> GAEVGRLRYPPEMPGAEVKVYKKVDNVDLKLYIYKPADWKPADRRSAIVFFFGGGWQSGSPAQFRPQCEYFAGRGMVAMAADYRVGSRHNVKVADCVADAKSAIRWVRQHAAELGVDPQKIVASGGXAGGHLAACTVMVPDLEAPEEDHTISSQANAAILFNPVLILSREGLKDHVPRQDWEERLRERLGTEPKAVSPYHHIRAGLPPMIIFHGTADNTVPFETIRLFAEAMKKAGNRCELVPFEGAAHGFFNFGRGDNLAYQKTLELADEFLVEIGFLAPKGESQP

In order to facilitate the purification costs, we searched the ESTHER database for a thermophilic esterase, and identified the Esterase 2 from Thermogutta terrifontis (TtEst2) that has been previously structurally characterized, and presents an open active site that could ease protein engineering for further optimizations. The recombinant protein was purified, biochemically characterized, and its kinetic behavior towards different OPNA studied, before performing a structural analysis of its complexes formed when soaked in a racemic solution of the OPNA. Biophysical characterizations demonstrated that TtEst2 is a monomer in solution, with some polydispersity and good thermostability at physiological pH. We determined the bimolecular inhibition rate constants for five representative OPNA, namely tabun, sarin, cyclosarin, VX, and paraoxon, to estimate if this enzyme could scavenge them at a fast pace.

Continuing this characterization, we solved the structures of the tabun, cyclosarin, and paraoxon conjugates. For each of these structures, the mobile region 165–190 could not be reasonably modeled, despite the presence of multiple disconnected blobs in the Fo–Fc map, notably a peak of >4 σ at the location of the indole ring of Trp180 in the VX-TtEst2 structure. For paraoxon, the strong electron density peak at covalent distance of Ser126 was modeled as an ethylphosphoryl adduct. This is consistent with the loss of the ethyl group close to the His248 through the dealkylation “aging” mechanism of cholinesterases. As in all the previous structures, the additional peak of electron density in the vicinity of the three different adducts was modeled as small molecules, a phosphate with partial occupancy (0.7 and 0.75) for tabun-TtEst2 and cyclosarin-TtEst2, and a carbonate for paraoxon-TtEst2, depending on the respective shape (trigonal or tetrahedral) in the feature-enhanced maps. However, the active site of TtEst2 being largely open to the solvent, there are no residues that could stabilize the leaving groups of paraoxon and VX, which are in consequence freely moving in the solvent.> MYNGKDRAQNSYQPMYQRPMQVQGQQQAQSFVGKKNTIGSVHGKAPMLMANNDVFTIGPYRARKDRMRVSVLEKYEVIGYIAAGTYGKVYKAKRQINSGTNSANGSSLNGTNAKIPQFDSTQPKSSSSMDMQANTNALRRNLLKDEGVTPGRIRTTREDVSPHYNSQKQTLIK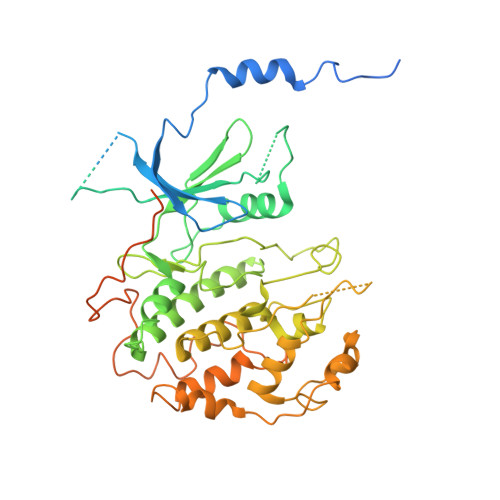KPLTVFYAIKKFKTEKDGVEQLHYTGISQSACREMALCRELHNKHLTTLVEIFLERKCVHMVYEYAEHDLLQIIHFHSHPEKRMIPPRMVRSIMWQLLDGVSYLHQNWVLHRDLKPANIMVTIDGCVKIGDLGLARKFHNMLQTLYTGDKVVVTIWYRAPELLLGARHYTPAVDLWSVGCIFAELIGLQPIFKGEEAKLDSKKTVPFQVNQLQRILEVLGTPDQKIWPYLEKYPEYDQITKFPKYRDNLATWYHSAGGRDKHALSLLYHLLNYDPIKRIDAFNALEHKYFTESDIPVSENVFEGLTYKYPARRIHTNDNDIMNLGSRTKNNTQASGITAGAAANALGGLGVNRRILAAAAAAAAAVSGNNASDEPSRKKNRR>[2x]GAMNWTVDIPIDQLPSLPPLPTDLRTRLDAALAKPAAQQPTWPADQALAMRTVLESVPPVTVPSEIVRLQEQLAQVAKGEAFLLQGGDCAETFMDNTEPHIRGNVRALLQMAVVLTYGASMPVVKVARIAGQYAKPRSADIDALGLRSYRGDMINGFAPDAAAREHDPSRLVRAYANASAAMNLVRALTSSGLASLHLV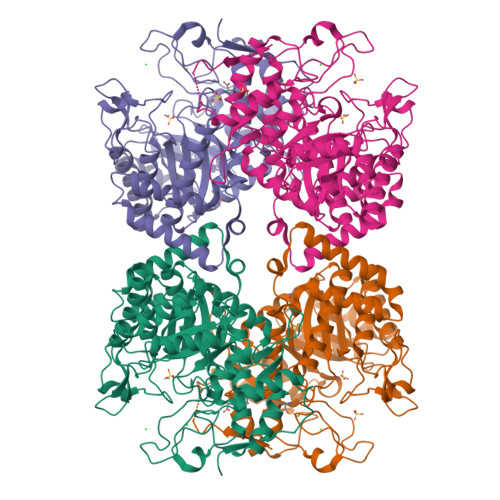HDWNREFVRTSPAGARYEALATEIDRGLRFMSACGVADRNLQTAEIYASHEALVLDYERAMLRLSDGDDGEPQLFDLSAHTVWIGERTRQIDGAHIAFAQVIANPVGVKLGPNMTPELAVEYVERLDPHNKPGRLTLVSRMGNHKVRDLLPPIVEKVQATGHQVIWQCDPMHGNTHESSTGFKTRHFDRIVDEVQGFFEVHRALGTHPGGIHVEITGENVTECLGGAQDISETDLAGRYETACDPRLNTQQSLELAFLVAEMLRD>GGTIAKVTG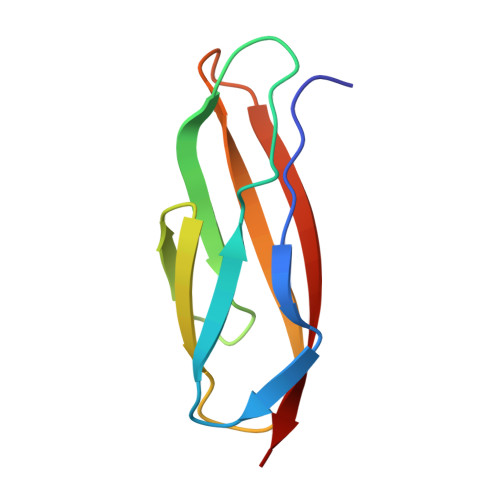PSTGAVGRNIEFSGKDSKDEDGKIVSYDWDFGDGATSRGKNSVHAYKKAGTYNVTLKVTDDKGATATESFTIEIKN[2x]> IIGGRESRPHSRPYMAYLQIQSPAGQSRCGGFLVREDFVLTAAHCWGSNINVTLGAHNIQRRENTQQHITARRAIRHPQYNQRTIQNDIMLLQLSRRVRRNRNVNPVALPRAQEGLRPGTLCTVAGWGRVSMRRGTDTLREVQLRVQRDRQCLRIFGSY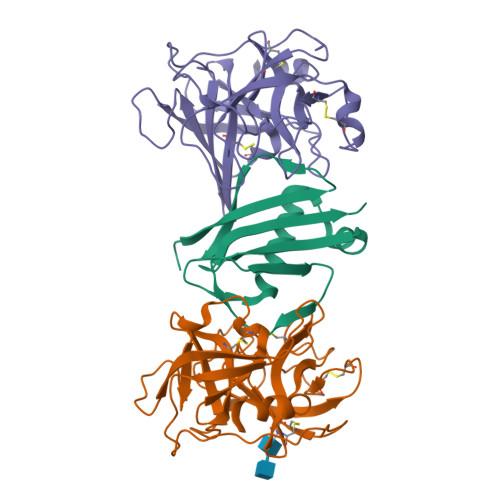DPRRQICVGDRRERKAAFKGDSGGPLLCNNVAHGIVSYGKSSGVPPEVFTRVSSFLPWIRTTMR;> IVGGRRARPHAWPFMVSLQLRGGHFCGATLIAPNFVMSAAHCVANVNVRAVRVVLGAHNLSRREPTRQVFAVQRIFENGYDPVNLLNDIVILQLNGSATINANVQVAQLPAQGRRLGNGVQCLAMGWGLLGRNRGIASVLQELNVTVVTSLCRRSNVCTLVRGRQAGVCFGDSGSPLVCNGLIHGIASFVRGGCASGLYPDAFAPVAQFVNWIDSIIQ;> GSTAEKDKLPATQKAKEMQNVPYTIAVDGIMAFNQSYLNLPKDSQLSYLDLGNKVKALLYDERGVTPEKIRNAKSAVYTITWKDGSKKEVDLKKDSYTANLFDSNSIKQIDINVKTK>HPETLVKVKDAEDQLGARVGYIELDLNSGKILESFRPEERFPLTSTFKVLLCGAVLSRVDAGQEQLGRRIHYSQNDLVEYSPVTEKHLTDGMTVRELCSAAITMSDNTAANLLLTTIGGPKELTAFLHNMGDHVTRLDRWEPELNEAIPNDERDTTMPAAMATTLRKLLTGELLTLASRQQLIDWMEADKVAGPLLRSALPAGWFIADKSGAGERGSRGIIAALGPDGKPSRIVVIYTTGSQATMDERN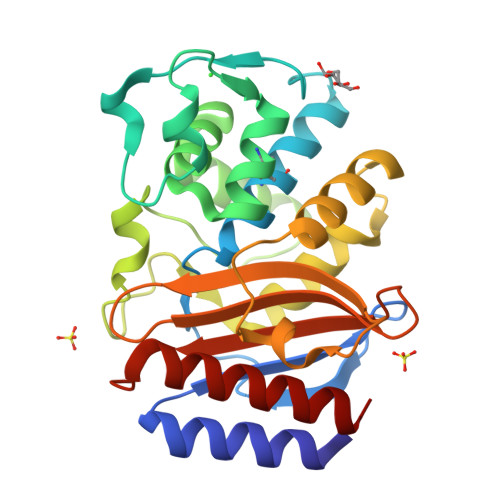RQIAEIGASLIKHW[2x]>[2x]GSKVMQKDVLAQ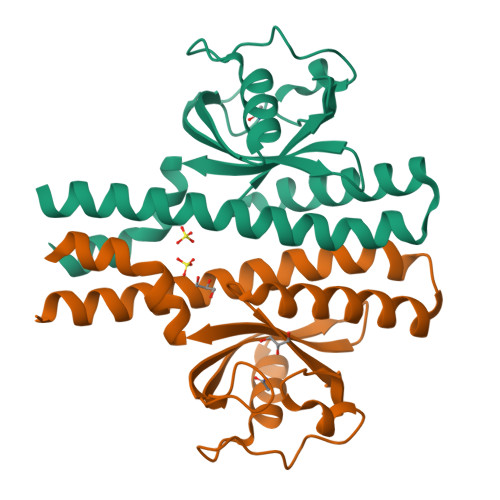LMEHLETGQYKKREKTLAYMTKILEQGIHEYYKSFDNDTARKMALDYFKRINDDKGMIYMVVVDKNGVVLFDPVNPKTVGQSGLDAQSVDGVYYVRGYLEAAKKGGGYTYYKMPKYDGGVPEKKFAYSHYDEVSQMVIAATSYYTDINTENKAIKEGVNKVFNENTTRL GlmM is a phosphoglucomutase enzyme catalyzing the conversion of glucosamine-6-phosphate to glucosamine-1-phosphate, which is subsequently used to produce the essential peptidoglycan precursor UDP-N-acetyl-glucosamine. CdaA (also referred to as DacA in some bacteria) is a membrane-bound cyclase with three predicted N-terminal transmembrane helices and a cytoplasmic catalytic DAC domain. c-di-AMP is formed from two molecules of ATP by enzymes containing a DAC domain. As part of the current study, we investigated how the activity the B. subtilis c-di-AMP cyclase CdaA is regulated by GlmM, a phosphoglucomutase enzyme required for the synthesis of an essential peptidoglycan precursor.

The GlmMF369 variant lacks the flexible C-terminal domain 4 and was constructed to aid subsequent structural investigations. On the other hand, diffracting crystals were obtained for the CdaACD:GlmMF369 complex, in which the GlmM protein lacks the flexible C-terminal domain 4. The crystals were obtained under two different conditions (see Experimental procedures section), and the structure of the CdaACD:GlmMF369 complex could be solved at 3.6 Å (Complex 1) and at 4.2 Å (Complex 2) by molecular replacement using the B. subtilis CdaACD and GlmM (dimer) structures as search models. While obtained under two different conditions, complex 1 and complex 2 were nearly identical and overlapped with an r.m.s.d. of 0.22 Å. Furthermore, in both complex structures, three complex molecules were obtained in the asymmetric unit and each complex was composed of a GlmMF369 dimer and a CdaACD dimer in the inactive dimer configuration. The three complexes obtained in the asymmetric unit were almost identical to each other, as indicated by the superposition r.m.s.d. of 0.15 to 0.20 Å for complex 1 and of 0.15 to 0.16 Å for complex 2. Since the obtained complex structures were basically identical, all further descriptions are based on the higher resolution complex 1 structure. In the complex, a CdaACD dimer was positioned in the large groove at the top of the GlmMF369 dimer and formed interactions with domain 2 of GlmM. Based on the atomic-resolution complex structure data, we suggest that GlmM inhibits the activity of CdaACD by preventing the formation of active head-to-head cyclase oligomers.

>MGKYFGTDGVRGVANSELTPELAFKVGRFGGYVLTKDKQRPKVLIGRDTRISGHMLEGALVAGLLSIGAEVMRLGVISTPGVSYLTKAMDAEAGVMISASHNPVQDNGIKFFGGDGFKLSDEQEAEIERLMDEPEDKLPRPVGADLGLVNDYFEGGQKYLQFLKQTADEDFTGIHVALDCANGATSSLATHLFADLDADVSTMGTSPNGLNINDGVGSTHPEALSAFVKEKNADLGLAFDGDGDRLIAVDEKGNIVDGDQIMYICSKHLKSEGRLKDDTVVSTVMSNLGFYKALEKEGIKSVQTAVGDRYVVEAMKKDGYNVGGEQSGHLIFLDYNTTGDGLLSAIMLMNTLKATGKPLSELAAEMQKF[6x];>[6x]EAQQKTIEAITKAINYMAKRRIGALLTIERDTGMGDYIETGIPLNAKVSSELLINIFIPNTPLHDGAVIMKNNEIAAAACYLPLSESPFISKELGTRHRAAVGISEVTDSLTIIVSEETGGVSVAKNGDLHRELTEEALKEMLEAEFKKNTRDTSSNRWYWRGKKNG>[60x]MWRVCARRAQNAAPRAGFGARWTAFREEPGAPCVTPQAGSALARCSSKTPGYGRVRALCGWSPVSRATPRNRVLLQLWGSPSRRWYSLPPHQKVPLPSLSPTMQAGTIARWEKKEGEKINEGELIAEVETDKATVGFESVEECYMAKILVAEGTRDVPVGAIICITVDKPEDVEAFKNYTLDSSAAPAPPAAPAPTPAAPAPSPTPSAQAPGSSYPTHMQVLLPALSPTMTMGTVQRWEKKVGEKLNEGDLLAEIETDKATIGFEVQEEGYLAKILIPEGTRDVPLGTPLCIIVEKEADIPAFADYRPAEVTDLKPPAPPPIPSPAAPVPPAPQ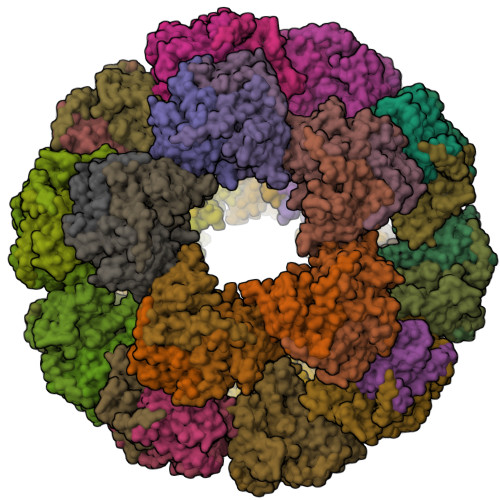PVAPPPSAPRPAAPAGPKGRVFVSPLAKKLAAEKGIDLTQVKGTGPDGRIIKKDIDSFVPTKAAPTPAAAVPPPSPGVAPVPTGVFTDIPISNIRRVIAQRLMQSKQTIPHYYLSIDVNMGEVLLVRKELNKMLEGKSKISVNDFIIKASALACLKVPEANSSWMDTVIRQNHVVDISVAVSTPAGLITPIVFNAHIKGLETIANDVVSLATKAREGKLQPHEFQGGTFTISNLGMFGIKNFSAIINPPQACILAIGASEDRLVPADNEKGFDVASMMSVTLSCDHRVVDGAVGAQWLAEFRKYLEKPITMLL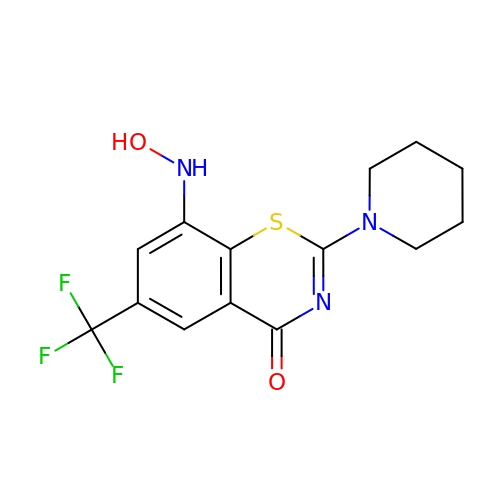8-(oxidanylamino)-2-piperidin-1-yl-6-(trifluoromethyl)-1,3-benzothiazin-4-one | C14 H14 F3 N3 O2 S | NFTFZGDVDRYPDT-UHFFFAOYSA-N(3~{S},6~{S})-3-[(3,5-dimethyl-4-oxidanyl-phenyl)methyl]-6-[(4-hydroxyphenyl)methyl]piperazine-2,5-dione 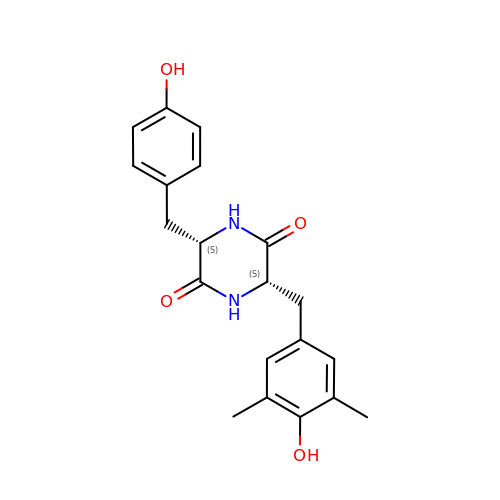| C20 H22 N2 O4 | UCEYENNEMBTPOB-IRXDYDNUSA-N2-[[3,4-bis(chloranyl)-5-methyl-1~{H}-pyrrol-2-yl]carbonylamino]-4-(2-morpholin-4-ylethoxy)-1,3-benzothiazole-6-carboxylic 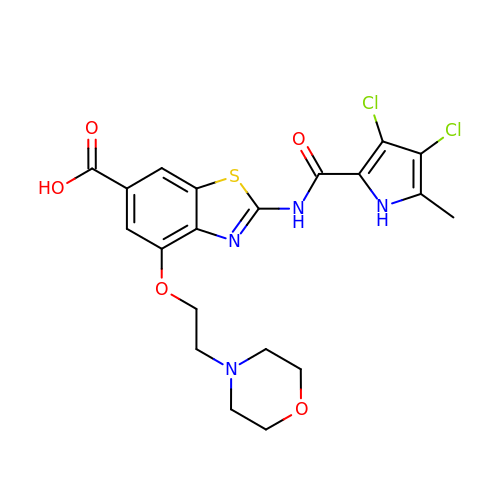acid | C20 H20 Cl2 N4 O5 S | IALGYKMHQTUZKU-UHFFFAOYSA-N> EKEK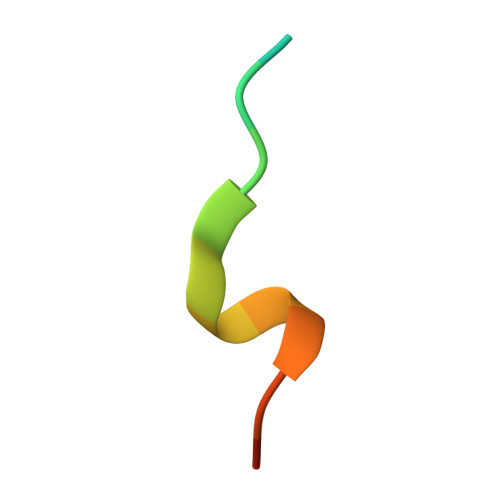QHDIRSFFVPQ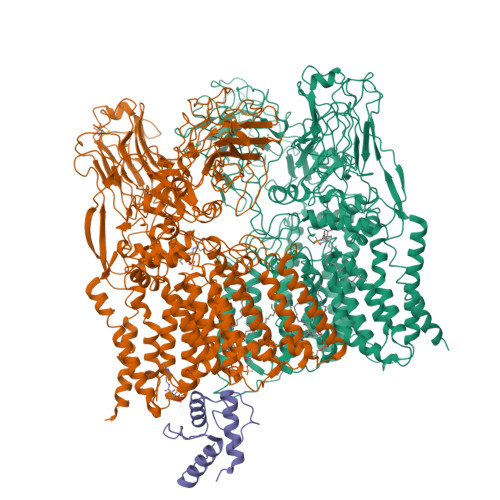> DYKDDDDKMTEPSRIARLIAVVAGIAGVLLCGLVPLLPVEETTATVLWPQGVGADGNVTELTAPLVAGAPRALDVTIPCRAVAELPADGGVVFSTNPAGGIEAGRNGMFIRANADVVYVAFRDTVAAVAPREAVDSGACSEIHVWADVSAVGADFAGIPDASGTLPVDKRPQVSGVFTDLKVPAQPGLAARIDIDTRFITSPTLLKTAVMVLGLACVIGSIVALALLDRGWRRRPPRTRGRAGLWTWITDTGVIGGLLIWHIVGAPTSDDGYNMTIARVASEAGYTTNYYRYFGASEAPFDWYQSVLSHLASISTAGVWMRLPATAAAIATWLIISRCVLPRIGRRVAANRVAMLTAGATFLAAWLPFNNGLRPEPLIAFAVITVWMLVENSIGTRRLWPAAVAIVIAMFSVTLAPQGLIALAPLLVGARAIGRVVTARRAGTGILASLAPLAASVAVVFVIIFRDQTLATVAESVRIKYVVGPTIPWYQEFLRYYFLTVEDSVDGSLTRRFAVLVLLLCLFGLIMVLLRRGRVPGAVSGPLWRLCGSTAIGLLLLILTPTKWAIQFGAFAGLAGALGGVTAFAFARVGLHSRRNLALYVTALLFILAWATSGLNGWFYVGNYGVPWFDKQPVIAHYPVTTIFLVLAIVGGLLAGWLHFRMDYAGHTEVADTGRNRALASTPLLIVATIMVVLELGSMVKATVGRYPVYTVGSANIAALRSAGDSCAMADAVLVEADPNEGMLQPVPGQRFGEYGPLGGEDPVGFTPNGVSDTLEPAEPVAANPGTPNSDGPVDKPNIGIGYAAGTGGGYGPEGVNGSRVFLPFGLDPSRTPVMGSYGENKLAAKATSAWYQLPPRTPDRPLVTVAAAGAIWYYEEDGSFNYGQSLKLQWGVHRPDGTYQALSEVQPIDIFQQKAWRNLRFPLAWAPPEANVARIVADDPNLSEDQWFAFTPPRVPVLQTAQQFLGSQTPVLMDIATAANFPCQRPFAERLGVAELPEYRIIPNFKQMVVSSNQWQSAADGGPFLFIQALLRTEAIPTYLRDDWYRDWGSIERYIRVVPQEQAPTAAIEEGSTRVFGWSRGGPIRALP;> MSGNMDEAVSGNMDEAVSAGKDVRIARWVATIAGLLGFVLSVSIPLLPVTQTTATLNWPQQGRLDNVTAPLISQAPLELTATVPCSVVRDLPPEGGLVFGTAPAEGRDAALNAMLVNVTETRVDVIVRNVVVASVNRDRVAGPDCQRIEITSNLDGTYADFVGLTQISGEDAGKLQRTGYPDPNLRPAIVGVFTDLTGPAPQGLSVSAEIDTRFTTHPTALKLAAMLLAIVSTVIALLALWRLDRLDGRRMHRLIPTRWRTVTAVDGVVVGGMAIWYVIGANSSDDGYILQMARTAEHAGYMANYFRWFGSPEDPFGWYYNVLALMTKVSDASIWIRLPDLICALICWLLLSREVLPRLGPAVAGSRAAMWAAGLVLLGAWMPFNNGLRPEGQIATGALITYVLIERAVTSGRLTPAALAITTAAFTLGIQPTGLIAVAALLAGGRPILRIVMRRRRLVGTWPLIAPLLAAGTVILAVVFADQTIATVLEATRIRTAIGPSQEWWTENLRYYYLILPTTDGAISRRVAFVFTAMCLFPSLFMMLRRKHIAGVARGPAWRLMGIIFATMFFLMFTPTKWIHHFGLFAAVGGAMAALATVLVSPTVLRSARNRMAFLSLVLFVLAFCFASTNGWWYVSNFGAPFNNSVPKVGGVQISAIFFALSAIAALWAFWLHLTRRTESRVVDRLTAAPIPVAAGFMVVVMMASMAIGVVRQYPTYSNGWANIRAFAGGCGLADDVLVEPDSNAGFLTPLPGAYGPLGPLGGEDPQGFSPDGVPDRIIAEAIRLNNPQPGTDYDWNRPIKLDEPGINGSTVPLPYGLDPKRVPVAGTYSTEAQQESRLSSAWYELPARDETERAAHPLVVITAAGTITGESVANGLTTGQTVDLEYATRGPDGTLVPAGRVTPYDVGPTPSWRNLRYPRSEIPDDAVAVRVVAEDLSLSQGDWIAVTPPRVPELQSVQEYVGSDQPVLMDWAVGLAFPCQQPMLHANGVTEVPKFRISPDYYAKLQSTDTWQDGINGGLLGITDLLLRASVMSTYLSQDWGQDWGSLRKFDTVVEATPAELDFGSQTHSGLYSPGPLRIRPHLGGIKAFHHHHHHHHHH;> MAATQEEIIAGLAEIIEEVTGIEPSEVTPEKSFVDDLDIDSLSMVEIAVQTEDKYGVKIPDEDLAGLRTVGDVVAYIQKLEEENPEAAAALREKFAADQ>MSIEKVPILGKETIHVGYGIADHIVREVIANLASSTYVIVTDTNMARTPQYSKLTDDFKTNLSEKRPESRLLTYCVSPGENNKNRATKAAVEDFLLQQGCTRDTVILAVGGGVIGDMIGFVAATFMRGVRVVQVPTTLLAMVDSSVGGKTAIDTPLGKNFIGAFHQPEYVFCDVSFLETLPARQFINGMAEVVKTAAIWNEEEFTRLENFSKKFLSVVTSKKPDLQSIKAELVKTVLESVRVKAGVVSSDEKEAGLRNLLNFGHTIGHAIEAVLTPEALHGECVSIGMIKEAELSRYLGILPPVAVARLSKCLVAYGLPVSIDDKEFLKKVGPKRHYVEIDILLKKMAIDKKNDGSKIRCVLLEKIGKCYQLKAHQVSKQDLSFVLTDEVLVHPFTNPPKENIIVPPGSKSISNRALILAALGNGTVRVKNLLHSDDTKHMLDAVASLKGAEISTEDNGETIVVKGNGGNLVTSGEELYLGNAGTASRFLTTVASLVGKSQASDDVILTGNARMQERPIGPLVDALGSNGSEIEYLNKQGSLPLKISAGNGLKGGRIELAATISSQYVSSILMCAPYAKEPVTLALVGGKPISQLYIDMTCAMMKSFGIEVTKSTTEEYTYHIPKGTYKNPSEYVIESDASSATYPLAFAAMTGTSCTIPNIGSSSLQGDAKFAVDVLKPMGCKVEQTTTSTTVTGPPRGHLKPLPHVDMEPMTDAFLTASVVAAVAKGGSSTSITGIANQRVKECNRIEAMVTELAKFGVPANELPDGIEIHGIDIEDLKTPEISKRGVSSYDDHRVAMSFSLLAGLCKEPVLILERSTTGKTWPGWWDILHSKFKIE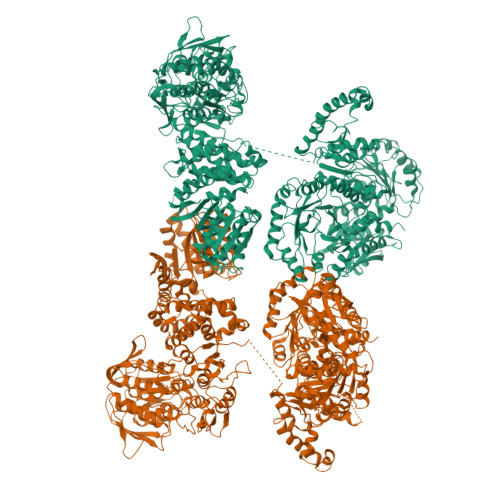LDGYEPPFNTDKHVDKSSDKSIIVIGMRGTGKSTLSEWLASFLGFKMLDMDKYLEEKLGTGIKSLIKAKGWEYFRQEEAIVAKECFTKFSKGYVLSTGGGIVEGEDARQQLKSYADNGGIVLHLHRDLDETVTFLAADTTRPAYSSEVQEVWLRREKWYHECSNYHFYSSHCSTEDEFNHLRRSFVNYIKLITGAERPVVPAGRSAAVVLTSPDLNEVVGDLESITIGADAVELRVDLFKDTSAEFVAAQIAVIRKHADLPIIYTVRTVSQGGKFPDENVDELKSLLLLGIRLGVAYVDLQLTAPNELIEEISSKKGFTRVIGTYQDINGELKWNNVEWKNKYNQGVSMNADIVRLVGKANSIQDNLDLENFKKQNTLKPLIAFNLGSQGKLSQVLNGTFTPISHKLLPNDEEFLTIGELNQTYFDIGGFTAKKFWVIGSPIEHSRSPNLHNAGYKALNLPYQFGRFEATDVDVVYDNLINKPDFGGLAITMPLKLDIMKFATKLSDAAETIGAVNTLIPIEGGYFGDNTDWVGISNSFIRAGVPPKSSSNGLVVGAGGTSRAAIYALHQMGCAKIYLVNRTAAKLEELVKSFPKDYNLEIVETEQQADKASKVSLAVSCIPADKPLDGEVLKKIERILSNGSEQSAGFKPTLLEASYKPRVTPIMKLTEEQYKWKVIPGVEMLVNQGDRQFKLHTGFTAPYEIIHRAVVEE[2x]> RIGRNEPCPCGSGK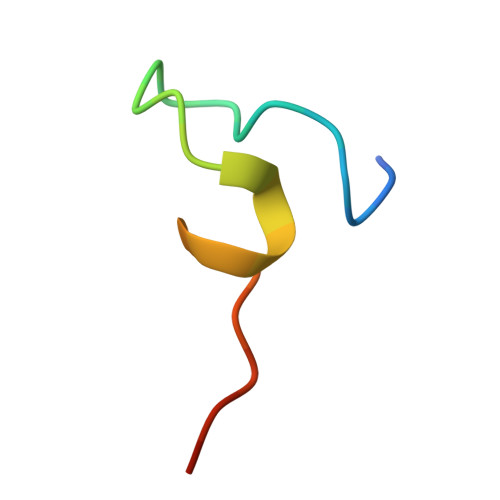KYKHCHGSRVARQ> MPLILLPAVNVVEGRAVRLVQGKAGSQTEYGSAVDAALGWQRDGAEWIHL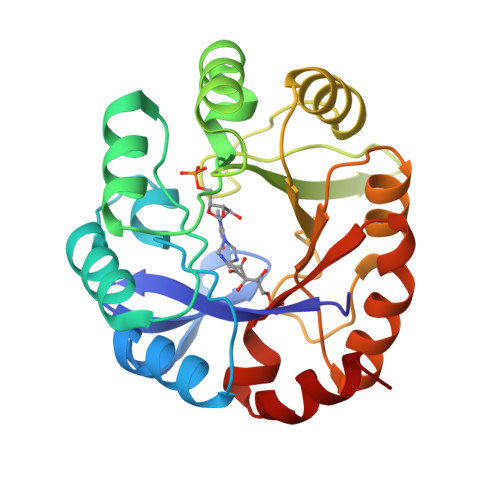VDLDAAFGRGSNHELLAEVVGKLDVQVELSGGIRDDESLAAALATGCARVNVGTAALENPQWCARVIGEHGDQVAVGLDVQIIDGEHRLRGRGWETDGGDLWDVLERLDSEGCSRFVVTDITKDGTLGGPNLDLLAGVADRTDAPVIASGGVSSLDDLRAIATLTHRGVEGAIVGKALYARRFTLPQALAAVRD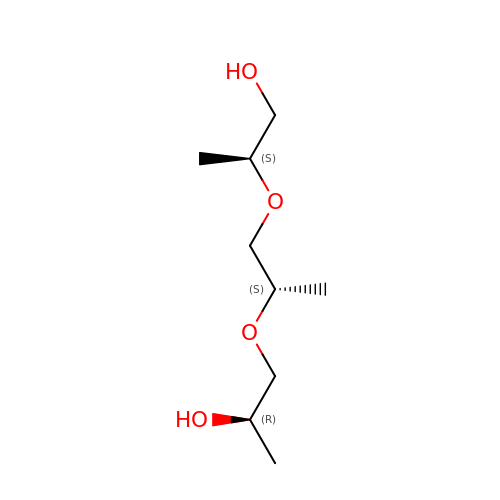(2S)-2-{[(2S)-2-{[(2R)-2-hydroxypropyl]oxy}propyl]oxy}propan-1-ol | C9 H20 O4 | LCZVSXRMYJUNFX-VGMNWLOBSA-N> NGIVPDAGHQGPDVSAVN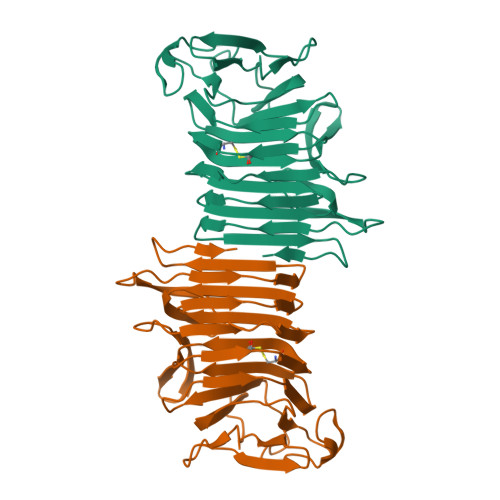GGTQVINIVTPNNEGISHNQYQDFNVGKPGAVFNNALEAGQSQLAGHLNANSNLNGQAASLILNEVVSRNPSFLLGQSEVFGIAAESVLSNPNGITCDGCGFINTSRSSLVVGNPLFENGQLKGYSTLNNTNLLSLGKNGLNTTGLLDLIAPRIDSRGKITAAEISAFTGQNTFSQHFDILSSQKPVSALDSYFFGSMQSGRIRIINTAEGSGVKLAGHHHHHH NADPH oxidases (NOX) are transmembrane proteins, widely spread in eukaryotes and prokaryotes, that produce reactive oxygen species (ROS). The cytosolic dehydrogenase (DH) domain belongs to the Ferredoxin NADP +Reductase (FNR) family which has motifs to bind a flavin cofactor and a pyridine dinucleotide NAD(P)H. Thus, the NOX core catalytic domain contains the necessary machinery to move electrons from the electron donor – NADPH – through the flavin and heme cofactors to the ultimate electron acceptor, molecular oxygen, to make the ROS product. SpNOX purifies as a monomer and is constitutively active, so it represents the minimal functional core shared by all NOX family members. Here, we obtained X-ray structures of WT and F397W mutant of DH-only, and of a F397W mutant of full-length SpNOX.

The use of the full-length SpNOX F397W construct resulted in about 20% of the crystals produced displaying diffraction limits close to 4 Å, with some crystals showing an anisotropic diffraction between 3 and 3.3 Å in a privileged direction of the crystals, as often observed for membrane proteins. The high-resolution model of the DH domain of SpNOX allowed resolution of the anisotropic crystals of full-length SpNOX-F397W to 3.6 Å. Like the previously reported structures of the NOX family, the crystallographic model of SpNOX harbors the N-terminal TM domain that encompasses 6 membrane-spanning alpha helices chelating two hemes, and the C-terminal cytosolic DH domain. The inner and outer heme are respectively coordinated by the imidazole rings of pairs of histidines H69 (TM3)/H129 (TM5) and H82 (TM3)/H142 (TM5), holding them perpendicular to the plane of the membrane. The metal-to-metal distance of the two hemes is ~21.5 Å, while the shortest interatomic distance is ~9.8 Å, between the vinyl groups. SpNOX has 9.2 Å edge-to-edge distance between the isoalloxazine ring to the inner heme; a conserved aromatic residue, Y136, at equal distance from both hemes (6.9 Å), or even F107 also on the pathway to the hemes, could assist the electron transfer between the hemes as previously suggested. We observed electronic density corresponding to the FAD cofactor at the interface of the DH and TM domain. FAD binding in the full-length construct preserves the π-stacking interaction with W397 and the interactions with F235 and P234 observed in the DH-only structure. In addition, the full-length SpNOX structure shows that the adenine extremity of FAD is packed in a pocket including the amino acid F399 from the DH domain– providing a potential role for this residue – as well as residues from the D-loop of the TM domain. Including SpNOX into this movement analysis is all the more interesting given that SpNOX is constitutively active. Here, Figure 8A shows that in our SpNOX structure, the relative position of TM vs DH domain is intermediate between the inactive (NOX2) and active (DUOX) structures.

> MEFSMKSVKGLLFIIASFILTLLTWMNTSPQFMIPGLALTSLSLTFILATRLPLLESWFHSLEKVYTVHKFTAFLSIILLIFHNFSMGGLWGSRLAAQFGNLAIYIFASIILVAYLGKYIQYEAWRWIHRLVYLAYILGLFHIYMIMGNRLLTFNLLSFLVGSYALLGLLAGFYIIFLYQKISFPYLGKITHLKRLNHDTREIQIHLSRPFNYQSGQFAFLKIFQEGFESAPHPFSISGGHGQTLYFTVKTSGDHTKNIYDNLQAGSKVTLDRAYGHMIIEEGRENQVWIAGGIGITPFISYIREHPILDKQVHFYYSFRGDENAVYLDLLRNYAQKNPNFELHLIDSTKDGYLNFEQKEVPEHATVYMCGPISMMKALAKQIKKQNPKTELIYEGWKFK> GSHMSSDSRYKRQVSGDEAYLEAAPLAELHAPAGMI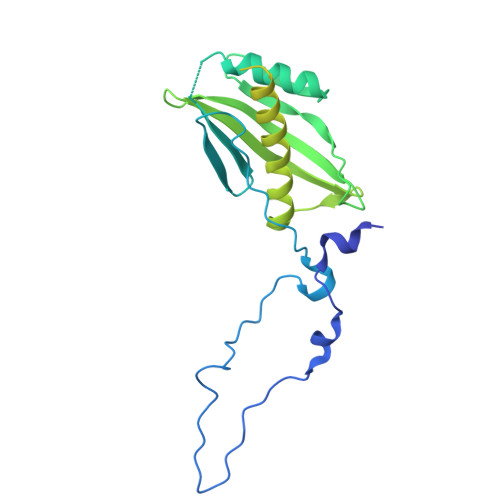LPVTSGDYAIPVTNGSGAVGKALDIRPPAQPLALVSGARTQFTGDTASLLVENGRGNTLWPQVVSVLQAKNYTITQRDDAGQTLTTDWVQWNRLDEDEQYRGRYQISVKPQGYQQAVTVKLLNLEQAGKPVADAASMQRYSTEMMNVISAGLDKSATDAANAAQNRASTTMDVQSAADDTGLPMLVVRGPFNVVWQRLPAALEKVGMKVTDSTRSQGNMAVTYKPLSDSDWQELGASDPGLASGDYKLQVGDLDNRSSLQFIDPKGHTLTQSQNDALVAVFQAAFSK>MTGNPDPNANPNVDPNANPNANPNANPNANPNANPNAEPSDKHIKEYLNKIQNSLSTEWSPCSVTCGNGIQVRIKPGSANKPKDELDYANDIEKKICKMEKCSSVFNVVNSGGSGTENHKDDAVLLKHGWCEMLKGGVIMDVKSVEQAKIAEEAGAIGVMVLENIPSELRNKEGVARSVDPSKVEEIKKCVSINVLARVRIGHF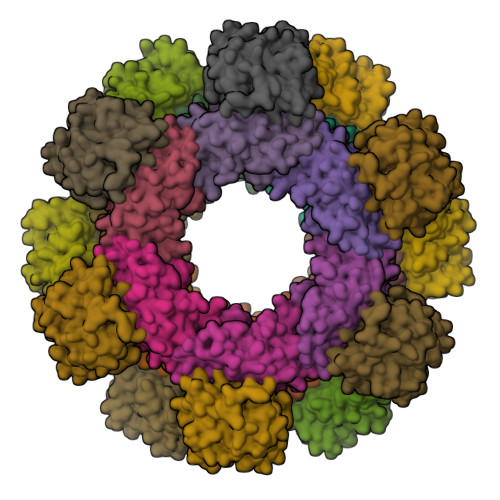VEAQILEELKIDMIDESEVLTIADEMHHIDKHKFKTPFVCGCTNLGEALRRISEGASMIRTKGEAGTGNIIEAIKHIRTVNNEICYLCCLSDSEVYHFAKKINAPIDLVLLTKKLKRLPVVNFAAGGVATPADAAMCMQLGMDGVFVGSGIFESENPRKMAASIVSAVSNFNNPKILLDVSMNLGKAMCGSTRVSDKWKNKNEEHTKFLTPQTGNPDPNANPNVDPNANPNANPNANPNANPNANPNAEPSDKHIKEYLNKIQNSLSTEWSPCSVTCGNGIQVRIKPGSANKPKDELDYANDIEKKICKMEKCSSVFNVVNSGGSLEHHHHHH[12x];>[12x]MTGNPDPNANPNVDPNANPNANPNANPNANPNANPNAEPSDKHIKEYLNKIQNSLSTEWSPCSVTCGNGIQVRIKPGSANKPKDELDYANDIEKKICKMEKCSSVFNVVNSGGSGTEITIGVLSLQGDFEPHINHFIKLQIPSLNIIQVRNVHDLGLCDGLVIPGGESTTVRRCCAYEQDTLYNALVHFIHVLKKPIWGTCAGCILLSKNVENIKLYSNFGNKFSFGGLDITICRNFYGSQQDSFICSLNIISDSSAFKKDLTAACIRAPYIREILSDEVKVLATFSHESYGPNIIAAVEQNNCLGTVFNPELLPHTAFQQYFYEKVKNYKYSTGNPDPNANPNVDPNANPNANPNANPNANPNANPNAEPSDKHIKEYLNKIQNSLSTEWSPCSVTCGNGIQVRIKPGSANKPKDELDYANDIEKKICKMEKCSSVFNVVNSGGSLEHHHHHH>[4x]MDPEFTNLIHFQSTEGKIWLGEQRMLLLQVSAMASFRREMVNTLGIERAKGFFLRQGYQSGLKDAELARKLRPNASEYDMFLAGPQLHSLKG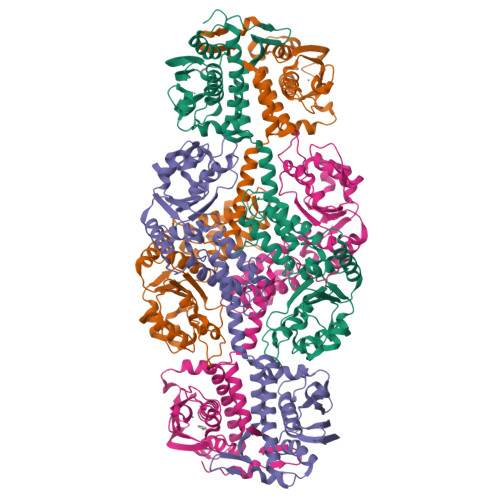LVKVRPTEVDIDKESGRFYAEMEWIDSFEVEISQTDLGQMQDPVCWTLLGYACAYSSAFMGREIIFKEVSCRGCGGDKCRVIGKPAEEWDDVASFKQYFKNDPIIEELYELQSQLVSLRTNLDKQEGQYYGIGQTPAYQTVRNMMDKAAQGKVSVLLLGETGVGKEVIARSVHLRSKRAAEPFVAVNCAAIPPDLIESELFGVEKGAFTGATQSRMGRFERADKGTIFLDEVIELSPRAQASLLRVLQEGELERVGDNRTRKIDVRVIAATHEDLAEAVKAGRFRADLYYRLNVFPVAIPALRERREDIPLLVEHFLQRFHQEYGKRTLGLSDKALEACLHYSWPGNIRELENVIERGIILTDPNESISVQALFPRA>[3x]GSSLEDPLRSFVRV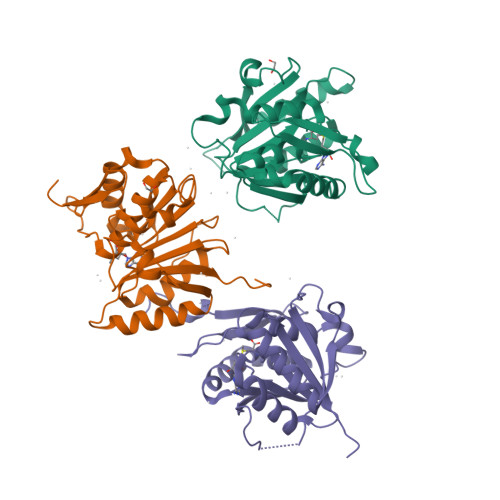LEKRDGTVLRLQQYSSGGVGCVVWDAAIVLSKYLETPEFSGDGAHALSRRSVLELGSGTGAVGLMAATLGADVVVTDLEELQDLLKMNINMNKHLVTGSVQAKVLKWGEEIEGFPSPPDFILMADCIYYEESLEPLLKTLKDISGFETCIICCYEQRTMGKNPEIEKKYFELLQLDFDFEKIPLEKHDEEYRSEDIHIIYIRKKKSKFPS>MIILFRGHMRDNSTEHKTRRAASSKDVRPAELDEVDRRILSLLHGDARMPNNALADTVGIAPSTCHGRVRRLVDLGVIRGFYTDIDPVAVGLPLQAMISVNLQSSARGKIRSFIQQIRRKRQVMDVYFLAGADDFILHVAARDTEDLRSFVVENLNADADVAGTQT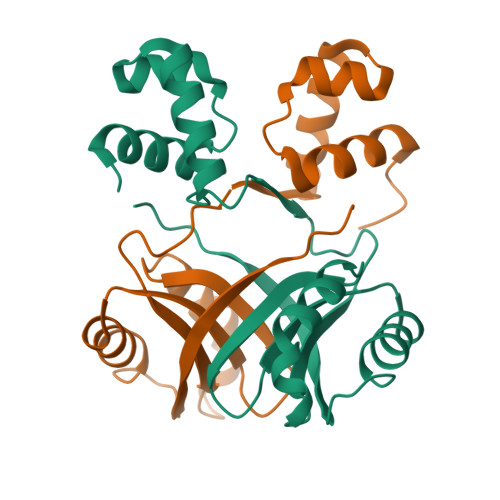SLIFEHLRGAAPIAAALGHHHHHH[4x]>[2x]RFLKVKNWETDVVLTDTLHLKSTLETGCTEHICMGSIMLPSQHTRKPEDVRTKDQLFPLAKEFLDQYYSSIKRFGSKAHMDRLEEVNKEIESTSTYQLKDTELIYGAKHAWRNASRCVGRIQWSKLQVFDARDCTTAHGMFNYICNHVKYATNKGNLRSAITIFPQRTDGKHDFRVWNSQLIRYAGYKQPDGSTLGDPANVQFTEICIQQGWKAPRGRFDVLPL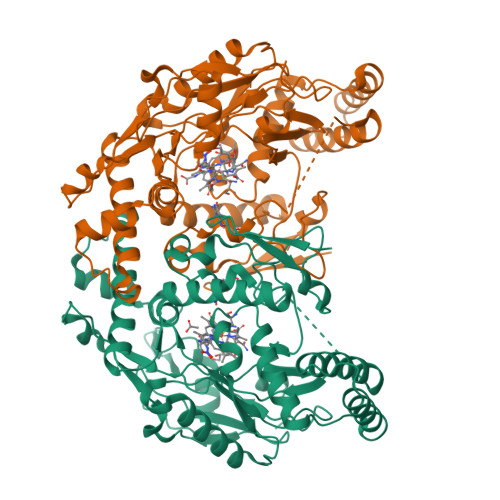LLQANGNDPELFQIPPELVLEVPIRHPKFDWFKDLGLKWYGLPAVSNMLLEIGGLEFSACPFSGWYMGTEIGVRNYCDNSRYNILEEVAKKMDLDMRKTSSLWKDQALVEINIAVLYSFQSDKVTIVDHHSATESFIKHMENEYRCRGGCPADWVWIVPPMSGSITPVFHQEMLNYRLTPSFEYQPDPWNTHVWKG> IVGGTASVRGEWPWQVTLHTTSPTQRHLCGGSIIGNQWILTAAHCFYGVESPKILRVYSGILNQAEIKEDTSFFGVQEIIIHDQYKMAESGYDIALLKLETTVNYADSQRPICLPSKGDRNVIYTDCWVTGWGYRALRDKIQNTLQKAKIPLVTNEECQKRYRGHKITHKMICAGYREGGKDACKGDSGGPLSCKHNEVWHL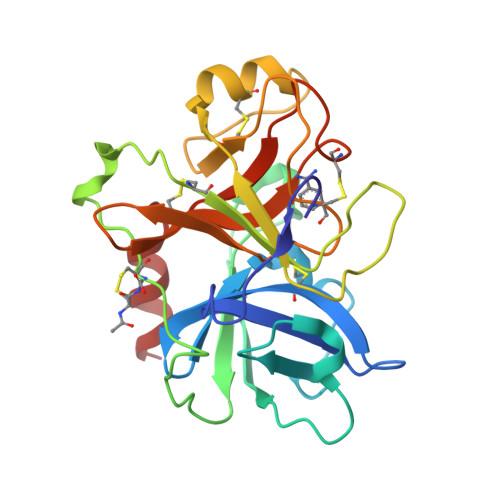VGITSWGEGCAQRERPGVYTNVVEYVDWILEKTQAV> TSWRLKDETYSYDGKLGADLKEEGKQVDLTLWSPSADKVSVVVYDKNDPDKVVGTVALEKGERGTWKQTLDSTNKLGITDFTGYYYQYQIERQGKTVLALDPYAKSLAAWNSDDSKIDDAHKVAKAAFVDPAKLGPQDLTYGKIHNFKTREDAVIYEAHVRDFTSDPAIAKDLTKPFGTFEA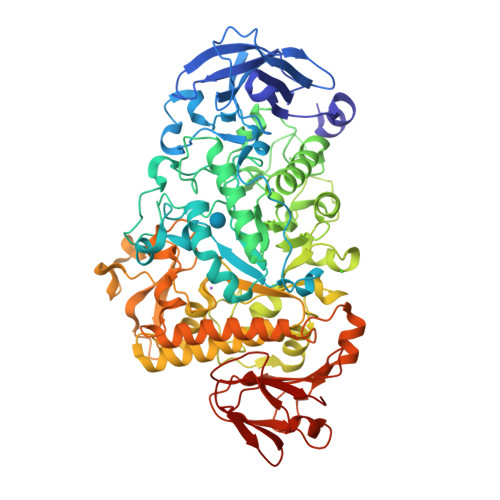FIEKLDYLKDLGVTHIQLLPVLSYYFVNELKNHERLSDYASSNSNYNWGYDPQNYFSLTGMYSSDPKNPEKRIAEFKNLINEIHKRGMGAILDVVYNHTAKVDLFEDLEPNYYHFMDADGTPRTSFGGGRLGTTHHMTKRLLIDSIKYLVDTYKVDGFRFDMMGDHDAASIEEAYKAARALNPNLIMLGEGWRTYAGDENMPTKAADQDWMKHTDTVAVFSDDIRNNLKSGYPNEGQPAFITGGKRDVNTIFKNLIAQPTNFEADSPGDVIQYIAAHDDLTLFDIIAQSIKKDPSKAENYAEIHRRLRLGNLMVLTAQGTPFIHSGQEYGRTKQFRNPAYRTPVAEDKVPNKSHLLRDKDGNPFDYPYFIHDSYDSSDAVNKFDWTKATDGKAYPENVKSRDYMKGLIALRQSTDAFRLKSLQDIKDRVHLITVPGQNGVEKEDVVIGYQITAPNGDIYAVFVNADEKAREFNLGTAFAHLRNAEVLADENQAGPVGIANPKGLEWTEKGLKLNALTATVLRVSQN1-(2-methyl-4-phenyl-pyrimidin-5-yl)-3-[[2-(trifluoromethyl)phenyl]methyl]urea 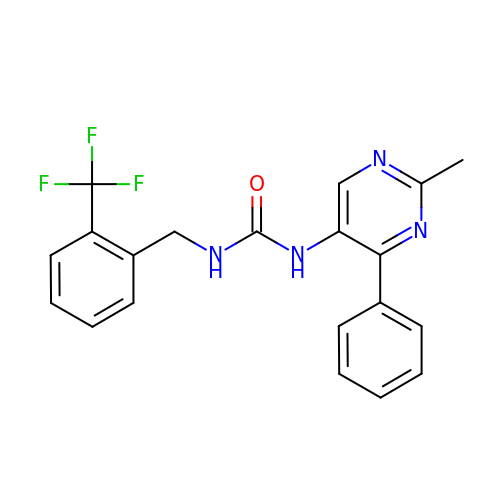| C20 H17 F3 N4 O | WEXHMXAXMQENNT-UHFFFAOYSA-N> MECFVPLRCDLDGSNIEQLRQSHLSRKFIIFDEQLNLWLWFQGNSQENKRFVLQNMIILINEAQVTRTSTIDDYFTQVENNENLWRLKNDCCSKILFKSNVVMNNGYNNQIKFVFEYKSVDANFNNQDSLQDPQAKYTLDKYSSEEILPSFEPVYSWSSAATKSSKNTNNHLEKNNRATHRVSSKNSEVHEADVSRNPNTFTLKLQYPIFSLLNMRLRNISLKSEHCILSSLDFQTSKASEQLTKKFIYPQEHNSFLKLNFQEISYKLIDGTSQI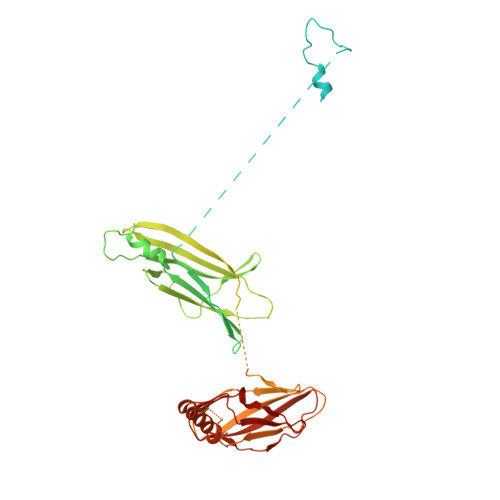ELDPICPLKVPLTAFSYDSISATFKLVLLPKSTQPHRVKITLAYELELHPNLKLPVRTSWETEVTLKRSMPISSTSSQYSSNNNNTNHSASFNGAANNVNSGGLANLRLGGVSSSRFSLGAASTTSLVNSKLSNVKFKFINSNIKVIKGEKFTMRLQIINSSSSPLDLVVYYNNTINPIPSANNVRNSNGINNCGMNNGTIPNSPLTLENQYQLHNKYRKIAEGIILLSNDYKIPVVPPRETYFADLRFIGIMSGYYGTLSGLKVLDLNTNELIEVGNGASVLIQ> MPKLPRGLRFGADNEI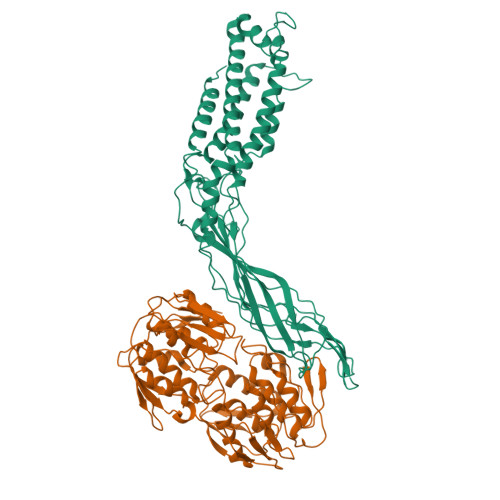LNDFQELWFPDLFIESSDTHPWYTLKGRVLNAHLDDRLPNVGGRQVRRTPHRVTVPIASSGLRPVTTVQYDPAALSFLLNARVDWDFGNGDSANLVINDFLFRTFAPKEFDFSNSLVPRYTQAFSAFNAKYGTMIGEGLETIKYLGLLLRRLREGYRAVKRGDLRALRRVIQSYHNGKWKPATAGNLWLEFRYGLMPLFYDIRDVMLDWQNRHDKIQRLLRFSVGHGEDYVVEFDNLYPAVAYFKLKGEITLERRHRHGISYANREGYAVFDNGSLRPVSDWKELATAFINPHEVAWELTPYSFVVDWFLNVGDILAQQGQLYHNIDIVDGFDRRDIRLKSFTIKGERNGRPVNVSASLSAVDLFYSRLHTSNLPFATLDLDTTFSSFKHVLDSIFLLTQRVKR;> MDKFRVQGPTKLQGEVTISGAKNAALPILFAALLAEEPVEIQNVPKLKDVDTSMKLLSQLGAKVERNGSVHIDARDVNVFCAPYDLVKTMRASIWALGPLVARFGQGQVSLPGGCTIGARPVDLHISGLEQLGATIKLEEGYVKASVDGRLKGAHIVMDKVSVGATVTIMCAATLAEGTTIIENAAREPEIVDTANFLITLGAKISGQGTDRIVIEGVERLGGGVYRVLPDRIETGTFLVAAAISRGKIICRNAQPDTLDAVLAKLRDAGADIEVGEDWISLDMHGKRPKAVNVRTAPHPAFPTDMQAQFTLLNLVAEGTGFITETVFENRFMHVPELSRMGAHAEIESNTVICHGVEKLSGAQVMATDLRASASLVLAGCIAEGTTVVDRIYHIDRGYERIEDKLRALGANIERVKGE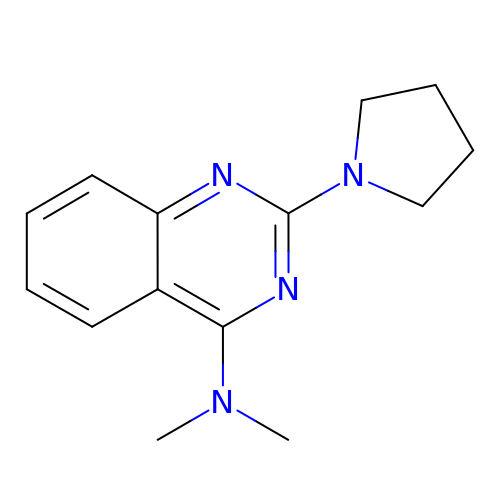~{N},~{N}-dimethyl-2-pyrrolidin-1-yl-quinazolin-4-amine | C14 H18 N4 | VONNLDQOEHSECV-UHFFFAOYSA-N> GLTNRLNATSNYSEYSLSVAVLADSEIENVTQLTSVTAPTGTDNENIQKLLADIKSSQNTDLTVNQSSSYLAAYKSLIAGETKAIVLNSVFENIIELEYPDYASKIKKIYTKGFTKKVEAPKTSKNQSFNIYVSGIDTYGPISSVSRSDVNILMTVNRDTKKILLTTTPADAYVPIADGGNNQKDKLTHAGIYGVDSSIHTLENLYGVDINYYVRLNFTSFLKMIDLLGGVDVHNDQEFSALHGKFHFPVGNVHLDSEQALGFVRERYSLADGDRDRGRNQQKVIVAILQKLTSTEALKNYSTIINSLQDSIQTNVPLETMINLVNAQLESGGNYKVNSQDLKGTGRMDLPSYAMPDSNLYVMEIDDSSLA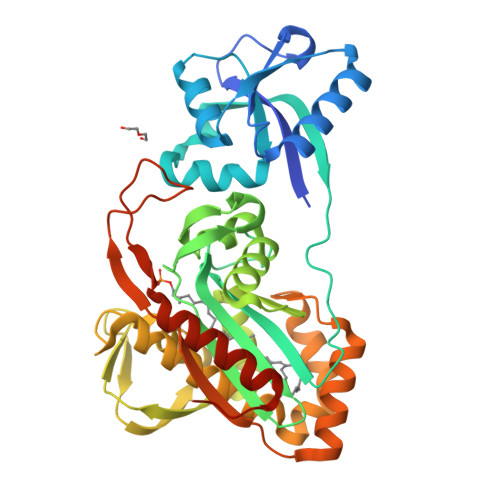VVKAAIQDVMEGRKLAAALEHHHHHH> MIVKHLEEIVDTKDDIDTTTWNSRRLLLTKDGMGFSLNDTLIKAGTETLIWYKNHVEAVYCIEGEGEIEVVGGETYPITPGMMYALDGHEKHYLRARSQMRMVC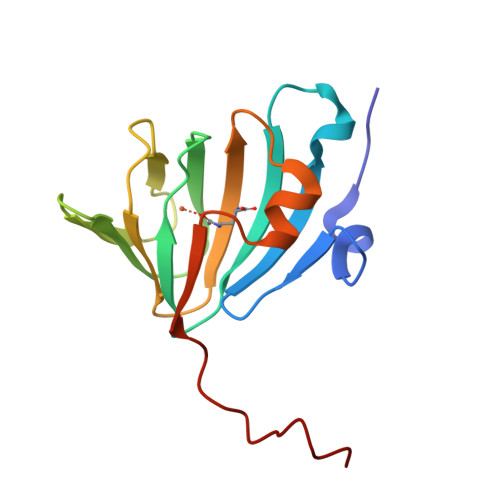VFNPPLTGAEVHDEEGTYPLLAPITDGSAWSHPQ>[2x]GEEEY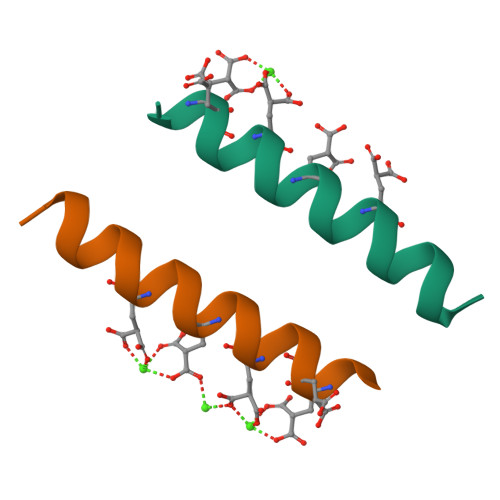QEMLENLREAEVKKNA> GPVEDAITAAIGRVADTVGTGPTNSEAIPALTAAETGHTSQVVPSDTMQTRHVKNYHSRSESTIENFLCRSACVYFTEYENSGAKRYAEWVITPRQAAQLRRKLEFFTYVRFDLELTFVITSTQQPSTTQNQDAQILTHQIMYVPPGGPVPDKVDSYVWQTSTNPSVFWTEGNAPPRMSVPFLSIGNAYSNFYDGWSEFSRNGVYGINTLNNMGTLYARHVNAGSTGPIKSTIRIYFKPKHVKAWIPRPPRLCQYEKAKNVNFQPSGVTTTRQSITTMTNT;> SPTVEECGYSDRVRSITLGNSTITTQECANVVVGYGVWPDYLKDSEATAEDQPTQPDVATCRFYTLDSVQWQKTSPGWWWKLPDALSNLGLFGQNMQYHYLGRTGYTIHVQCNASKFHQGCLLVVCVPEAEMGCATLNNTPSSAELLGGDTAKEFADKPVASGSNKLVQRVVYNAGMGVGVGNLTIFPHQWINLRTNNSATIVMPYTNSVPMDNMFRHNNVTLMVIPFVPLDYCPGSTTYVPITVTIAPMCAEYNGLRLAGHQ;> GLPTMNTPGSCQFLTSDDFQSPSAMPQYDVTPEMRIPGEVKNLMEIAEVDSVVPVQNVGEKVNSMEAYQIPVRSNEGSGTQVFGFPLQPGYSSVFSRTLLGEILNYYTHWSGSIKLTFMFCGSAMAT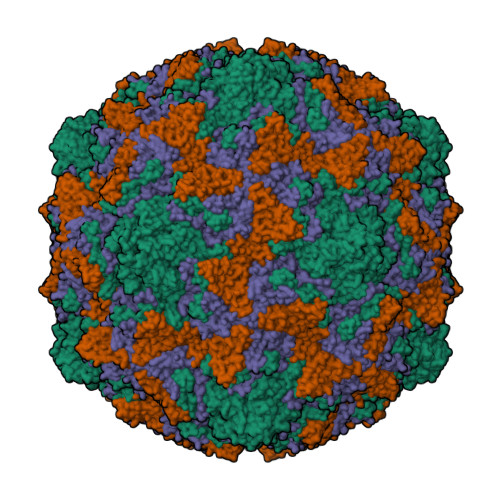GKFLLAYSPPGAGAPTKRVDAMLGTHVVWDVGLQSSCVLCIPWISQTHYRYVASDEYTAGGFITCWYQTNIVVPADAQSSCYIMCFVSACNDFSVRLLKDTPFISQENFFQ;> GAQVSTQKTGAHETGLNASGNSIIHYTNINYYKDAASNSANRQDFTQDPSKFTEPVKDIMIKSLPALN> MGSSHHHHHHSQDPMNILLVSQCEKRALSETRRILDQFAERRGERTWQTPITQAGLDTLRRLLKKSARRNTAVACHWIRGRDHSELLWIVGDASRFNAQGAVPTNRTCRDILRKEDENDWHSAEDIRLLTVMAALFHDIGKASQAFQAKLRNRGKPMADAYRHEWVSLRLFEAFVGPGSSDEDWLRRLADKRETGDAWLSQLARDDRQSAPPGPFQKSRLPPLAQAVGWLIVSHHRLPNGDHRGSASLARLPAPIQSQWCGARDADAKEKAACWQFPHGLPFASAHWRARTALCAQSMLERPGLLARGPALLHDSYVMHVSRLILMLADHHYSSLPADSRLGDPNFPLHANTDRDSGKLKQRLDEHLLGVALHSRKLAGTLPRLERQLPRLARHKGFTRRVEQPRFRWQDKAYDCAMACREQAMEHGFFGLNLASTGCGKT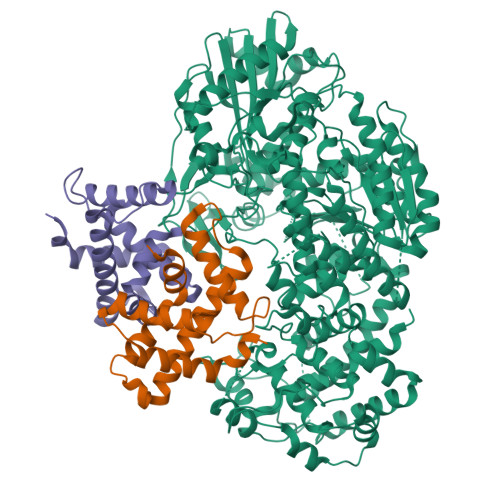LANGRILYALADPQRGARFSIALGLRSLTLQTGQAYRERLGLGDDDLAILVGGSAARELFEKQQERLERSGSESAQELLAENSHVHFAGTLEDGPLREWLGRNSAGNRLLQAPILACTIDHLMPASESLRGGHQIAPLLRLMTSDLVLDEVDDFDIDDLPALSRLVHWAGLFGSRVLLSSATLPPALVQGLFEAYRSGREIFQRHRGAPGRATEIRCAWFDEFSSQSSAHGAVTSFSEAHATFVAQRLAKLEQLPPRRQAQLCTVHAAGEARPALCRELAGQMNTWMADLHRCHHTEHQGRRISFGLLRLANIEPLIELAQAILAQGAPEGLHVHLCVYHSRHPLLVRSAIERQLDELLKRSDDDAAALFARPTLAKALQASTERDHLFVVLASPVAEVGRDHDYDWAIVEPSSMRSIIQLAGRIRRHRSGFSGEANLYLLSRNIRSLEGQNPAFQRPGFETPDFPLDSHDLHDLLDPALLARIDASPRIVEPFPLFPRSRLVDLEHRRLRALMLADDPPSSLLGVPLWWQTPASLSGALQTSQPFRAGAKERCYALLPDEDDEERLHFSRYEEGTWSNQDNLLRNLDLTYGPRIQTWGTVNYREELVAMAGREDLDLRQCAMRYGEVRLRENTQGWSYHPYLGFKKYN;>[2x]MSNTISDRIVARSVIEAARFIQSWEDADPDSLTEDQVLAAAGFAARLHEGLQATVLQRLVDESNHEEYREFKAWEEALLNADGRVASSPFADWGWWYRIANVMLATASQNVGVTWGSRVHGRLMAIFQDKFKQRYEEQA> SSASAAAAAAAAALAAGAADGPTNDEAPGADGRRSYINLPAHHSAIIQQWVLDAGSGSILGHVNGGFLPNPVAAHSGSEFALASTSFSRIAKGKRTDYVEVFDPVTFLPIADIELPDAPRFDVGPYSWMNANTPNNADLLFFQFAAGPAVGLVVQGGSSDDQLLSSPTCYHIHPGAPSTFYLLCAQGGLAKTDHAGGAAGAGLVGAMLTAAQNLLTQPAQANKSGRIVWPVYSGKILQADISAAG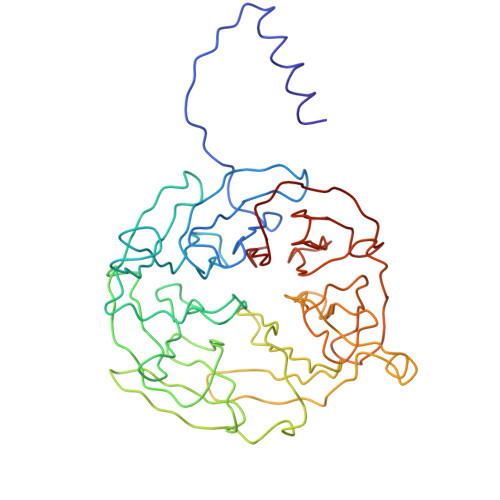ATNKAPIDALSGGRKADTWRPGGWQQVAYLKSSDGIYLLTSEQSAWKLHAAAKEVTSVTGLVGQTSSQISLGHDVDAISVAQDGGPDLYALSAGTEVLHIYDAGAGDQDQSTVELGSGPQVLSVMNEA>MNNKGSGLTPAQALDKLDALYEQSVVALRNAIGNYITSGELPDENARKQGLFVYPSLTVTWDGSTTNPPKTRAFGRFTHAGSYTTTITRPTLFRSYLNEQLTLLYQDYGAHISVQPSQHEIPYPYVIDGSELTLDRSMSAGLTRYFPTTELAQIGDETADGIYHPTEFSPLSHFDARRVDFSLARLRHYTGTPVEHFQPFVLFTNYTRYVDEFVRWGCSQILDPDSPYIALSCAGGNWITAETEAPEEAISDLAWKKHQMPAWHLITADGQGITLVNIGVGPSNAKTICDHL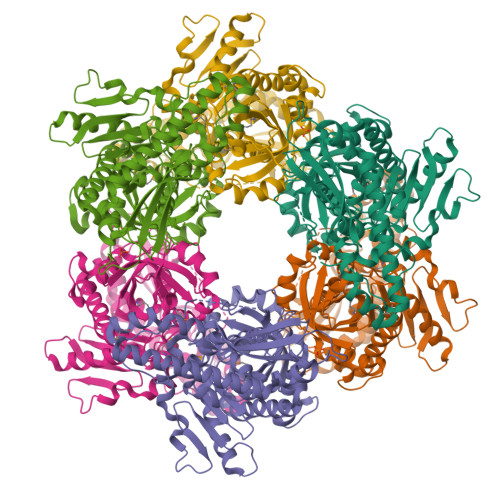AVLRPDVWLMIGHCGGLRESQAIGDYVLAHAYLRDDHVLDAVLPPDIPIPSIAEVQRALYDATKLVSGRPGEEVKQRLRTGTVVTTDDRNWELRYSASALRFNLSRAVAIDMESATIAAQGYRFRVPYGTLLCVSDKPLHGEIKLPGQANRFYEGAISEHLQIGIRAIDLLRAEGDRLHSRKLRTFNEPPFR[6x]>[2x]M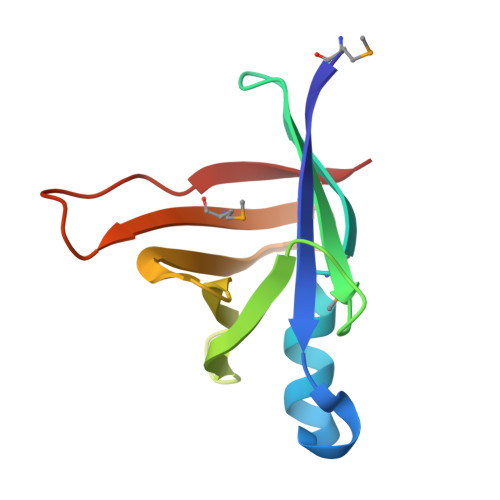YQLQFINLVYDTTKLTHLEQTNINLFMGNWSNHQLQKSICIRHGDDTSHNQYHILFIDTAHQRIKFSSIDNEEIIYILDYDDTQHILMQTSSKQGIGTSRPIVYERLV>[2x]GSHMGPSLDFALSLLRRNVRQVQTDQGHFTMLGVRDRLAVLPRHSQPGKTIWIEH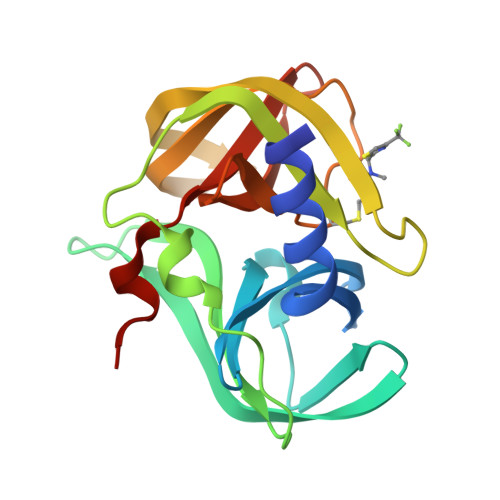KLVNVLDAVELVDEQGVNLELTLITLDTNEKFRDITKFIPENISTASDATLVINTEHMPSMFVPVGDVVQYGFLNLSGKPTGRTMMYNFPTKAGQCGGVVTSVGKIIGIHIGGNGRQGFCAGLKRSYFASEQ> GPGHMVVKFSYMWTINNFSFCREEMGEVIKSSTFSSGANDKLKWCLRVNPKGLDEESKDYLSLYLLLVSCPKSEVRAKFKFSIL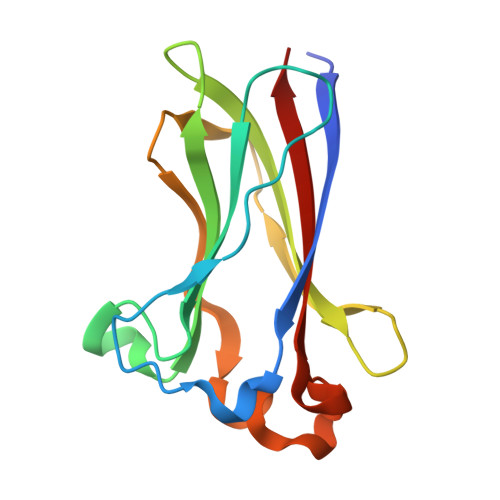NAKGEETKAMESQRAYRFVQGKDWGFKKFIRRGFLLDEANGLLPDDKLTLFCEVSVVQD>[2x]MKYSQCLKGEVVMIPALAKKILHVTVGTLLVSSAASMMVYLNSMCHMAANSKTQQIQGDDNKDDKFPLAAISKVVTTLWAVDRLGPDYRFKTKLHVTPTANGSYDIHIEGSRDPLFGRNMSYFLISELNRMKITKIEKLTFDENFLLAWLAEEKPMIGGTTPKYDTVEQQASIVRATLTSSFATAISPGYYTILKTKAARIGVQMSNRPKIDVRTISFVKKAEFQKNEKSTTMVLMSAPLKTILKRMNNQSNNYIADNLYWNLGGTEAFNAYIAGKMQADTSDIEFHNGSGNNEGSVAKPVYNEATCEMMIKVLYSLDKSLSAKGYDLSDVMAVAAKDKASTVGSYGGVMAGSTTAKTGSVNKAKTLMGSVSTKNGEIYFAVLMHTDYDKSRSDWGVASQQIKNKVSQLINQNGGPKAIKYTEQLPLPFDKYSYLTKANTITTEKK

Here we show that Bdellovibrio bacteriovorus utilizes a small ankyrin repeat protein, Bd3460, to protect itself from endopeptidase activities during entry of prey. We demonstrate that endopeptidase complexation by Bd3460 prevents cell wall decrosslinking, and that both the Bd0816 and Bd3459 targets bind this self-protection protein via a common epitope. Previously, we assigned prey cell rounding to the action of two secreted Bdellovibrio peptidoglycan DD-endopeptidases, Bd0816 and Bd3459, that act to modify the invaded cell wall via hydrolysis of the structural 3-4 peptide crosslinks6. In summary, we conclude that we have identified and characterized the first ever self-protection protein encoded by predatory bacteria—ankyrin repeat protein Bd3460 from Bdellovibrio inhibits the prey wall decrosslinking enzymes Bd3459/Bd0816 and in doing so protects the predator from the shape transition that this catalyses in prey.

Structure and activity analyses of DD-endopeptidase Bd3459 revealed a highly active enzyme with an open active site adapted for prey peptidoglycan diversity, rather than self-wall maintenance (this was also inferred for the homologous Bd0816). We next utilized a modified version of our original Bd3459 construct (starting post signal peptide with K38 mutated to become the new N-terminal methionine) that represents a more ‘native' signal peptide-processed form of the DD-endopeptidase6. Upon comparison with our structures of the uncomplexed proteins, Bd3459 does not alter in conformation upon binding, whereas Bd3460 undergoes further flexation around the region between AR4-AR5.10-[2-[(3~{R})-1-methyl-3-oxidanyl-2-oxidanylidene-pyrrolidin-3-yl]ethynyl]-~{N}3-(oxan-4-yl)-5,6-dihydroimidazo[1,2-d][1,4]benzoxazepine-2,3-dicarboxamide 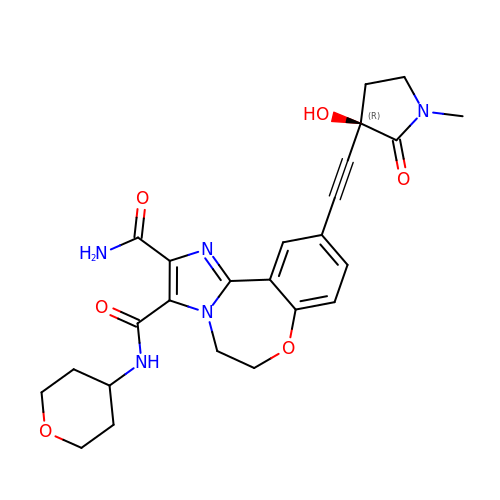| C25 H27 N5 O6 | ZGTZKIXFBFZCBL-VWLOTQADSA-N> MEMMIKKRIKQVKKGDQDAFADIVDIYKDKIYQLCYRMLGNVHEAEDIAQEAFIRAYVNIDSFDINRKFSTWLYRIATNLTIDRIRKKKPDYYLDAEVAGTEGL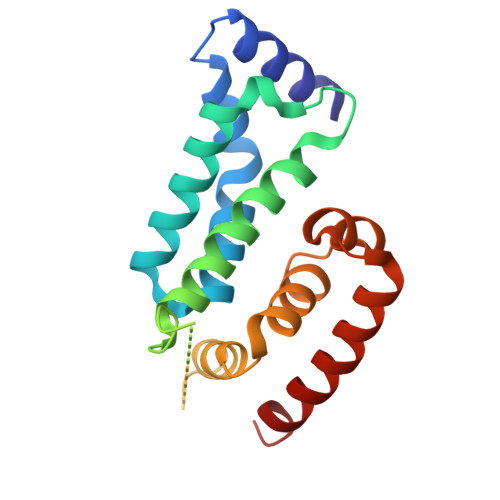TMYSQIVADGVLPEDAVVSLELSNTIQQKILKLPDKYRTVIVLKYIDELSLIEIGEILNIPVGTVKTRIHRGREALRKQLRDL>[12x]GYIQERLKSLNDIETQLCSMLQ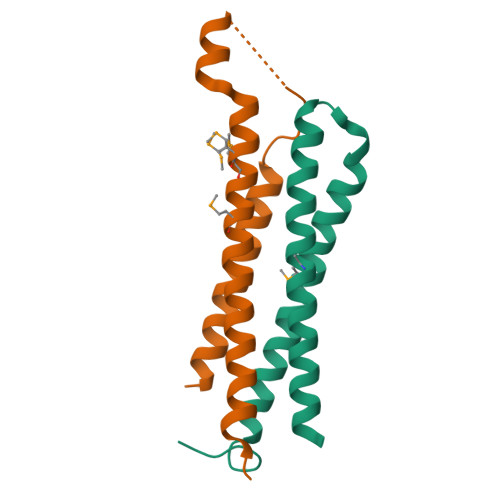EASQVTFIFGELKRGNESVKPQFENHVKQFYERLDKSTTQLRKEIQLLDENVGTRLLPINVNKK;>GSHMSNQALYEKLEQTRTILSVKLAELINITTIADRNDDDEGSFAQENSELAVATTSVMMVNNQTMQLIKNVQDLLILTRSIKEKWLLNQIP[12x]> MAPKDNTWYTGAKLGWSQYHDTGLINNNGPTHENKLGAGAFGGYQVNPYVGFEMGYDWLGRMPYKGSVENGAYKAQGVQLTAKLGYPITDDLDIYTRLGGMVWRADTYSNVYG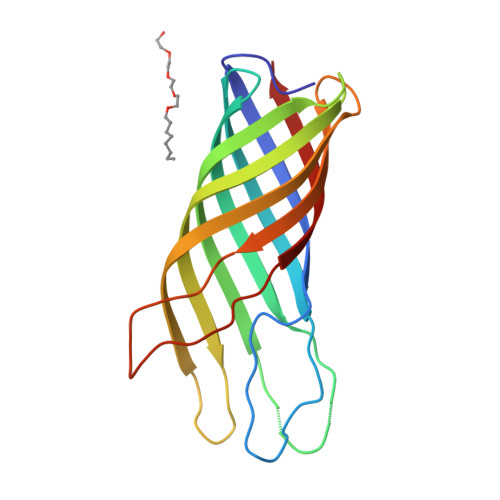KNHDTGVSPVFAGGVEYAITPEIATRLEYQWTNNIGDAHTIGTRPDNGMLSLGVSYRFG>GSMPPQLHNGLDFSAKVIQGSLDSLPQEVRKFVEGNAQLCQPEYIHICDGSEEEYGRLLAHMQEEGVIRKLKKYDNCWLALTDPRDVARIESKTVIITQEQRDTVPIPKSGQSQLGRWMSEEDFEKAFNARFPGCMKGRTMYVIPFSMGPLGSPLAKIGIELTDSPYVVASMRIMTRMGTSVLEALGDGEFIKCLHSVGCPLPLKKPLVNNWACNPELTLIAHLPDRREIISFGSGYGGNSLLGKKCFALRIASRLAKEEGWLAEHMLILGITNPEGKKKYLAAAFPSACGKTNLAMMNPTLPGWKVECVGDDIAWMKFDAQGNLRAINPENGFFGVAPGTSVKTNPNAIKTIQKNTIFTNVAETSDGGVYWEGIDEPLAPGVTITSWKNKEWRPQDEEPCAHPNSRFCTPASQCPIIDPAWESPEGVPIEGIIFGGRRPAGVPLVYEALSWQHGVFVGAAMRSEATAGAEHKGKVIMHDPFAMRPFFGYNFGKYLAHWLSMAHRPAAKLPKIFHVNWFRKDKNGKFLWPG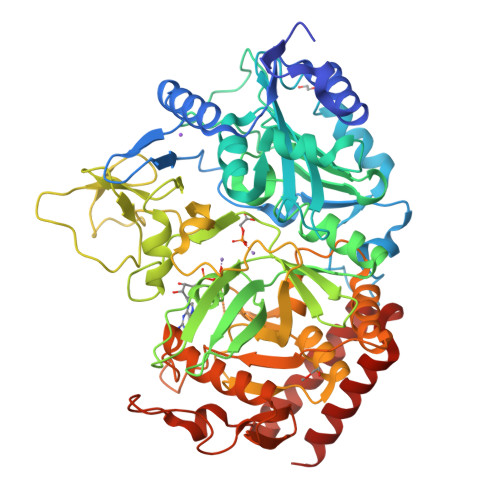FGENSRVLEWMFGRIEGEDSAKLTPIGYVPKEDALNLKGLGDVNVEELFGISKEFWEKEVEEIDKYLEDQVNADLPYEIERELRALKQRISQM[2x]>[2x]MNILKHFPSYVGPSKIRTLVIPIGHWTRKEFNNAVQKLSEFNEIHLSDVTPIDSPIFTPQGFPHGKLFFDFLTIDHDDALELFLYDFEPFRKTFVIIGLVNDYSDPLTNLNFMKEKYPTLISPNLVYASSTPTKELEQTIDTMENVFASSPDMQKNIETIMCDIARNFLTALNSYYSSYKHVTLRSPGAIGGNAVLKTTLIRQNSYTSSSSSTPMSAVQSSVSSSSKAGSVTTASKRLSSFEMTTNSLKRSASLKLATTLSTSENRSQQKSLGRQMKILGNFQLLAGRYVDALNSFVDAITTLYKVRDYLWLGSALDGISICFLLLSYLGLSYQIPQIVSLICPVEKLNFESSSTGISPVDSNSKATASTTASSTPRNSISIAAMQSPRNSIMSLSAPALNIDVENINLPLLIKCISDKVLYYYDLSLMHNSEYAPQVVYCEFLLKTLTFMTSCYKSSEFSKDVLDNIVKNQHRALSDIPNSPMFPRFEVYFYSNKLFELQLKEMQVEAQIKIYSTMAEVYRLLGYKRKQLFVLRLLMVALLATPNKIAWHPDYRTLIDTIIELLNINESEAKINVDDPSQSTWLILQKKILQLCIKVSRKINDFEYVAKFSSILITKYTHLLNQSEQDALFKEYIQPSITNESITSYWDPFILREVVINRILDSDPTSNEIPLESDVSSLESLENRQKTQDINPQEVFNPFKRVQPTSFVSNNSTKVPILVFLVGDKAEFTCRVQNPFKFDFTINDIQLDEEISEFCEIDRKAVSYSGPYNVKAESIRSITLPLIIKKPTYKKIYEISCLKISILKLPLQKFDIINDSRRSNPVEEEAEYSKCIYGKLKIKILPEQPQLELLSTSKMTRNSWMMLDGTKTDFHITVRNKSLSCAINHIKIIPMNNIEQMLKPDYWKKMPPDDLYIMEKQLDWLSKSCVRIIKLPTVIKPNETITFDLELDNTAVPFNFTGFDLLIEYGMSATDESCIYLKKLSIPYEVTLRRTIEVPSMDIIPLNELFSSQVENVDWIEYVMSKIRAESNLHSRDFILLLLDFRNSWIDGIKLNVQFEDFTSNEYHVEASHTSRIIVPIKKIDYKKYNFENTPIPRIYPGRQFIQSGLNEEQTIEMRQKFWCREHIISKLKCNWKLTTDQSVTGSVDFNKFIEKFDHKMVYTIYPGRLFYGVQLLLDEPKVKVGEIINLKIITEPTSTCRRKQNSTVNFLDIVIFDSKTSKILPRSNRRILYNGSLTKPISTTKVSEINLEIIPIEKGRYEFSVCISKSNNQDGIIQFDSENVILSVI;>MDKEIYCGSVPVSYFDPFDLFESLRPEFQQILPLDNIHWKAFDGTVRTVNRLPIELIPEGRGEADKSNDEQPFIRFLIVNCISIDQYRAKVRPLVRQWLPNLESVSSSTGEKMIYKPIILLYANSEVVDSNLFKSVSLMEKFGKDFPHVQTLEVRSVYRSPKERQEFWNQFSQKIKASVLSIFQKRLTHLQHSLANLQKGNNFEEQLLTREKLYELYVVFNILEDASLELQKIKKEILRRNMNMPDGKLQVPFESSSKSDESLGSIIIEGTLDKFQLHKYFFIRRLRLLKLEDQTLTAFVGAFQLIKNFIESISIEYRKSVRLLEFKHYFITSMLSYFEFENVSNPLLCEIKAELLMLKRDNWVQGVMATSGYRLMDKNYPNSDVKYKFDLLKETFVDETVFQENFLTLTKEILSLFNKCEGKRQRIVDILSIEIGLLYYQGKKYEEAVSLFLSCYEYYTQTNWNSIGLKILQVFIDSLSHCPKLDVLQIDGESVSASAVLTNAFLNILKLCKDNDSKEIWWKKFMDLQMKNNIHLMYPLDGLFEVTLNSKVHLARANVSAIEVNLKSYGFPEDISTKTMRLSLKNMGGDVIVFGASDFLLKKGENKLILECRDIMYGEFSLLSFEIIVEGITFVKEFPENQDEFIVVPEIYCKESTKVLVKQAHNLNLGEYALELKSVQSDALESLQVEVEVQKNIGNMKNLPVSFSMDEIQARKRYNTPFENVRLEYYLLDQITAFDLIIKTSFTKKNDQGTFGETKKVRIQCYLQLSVSVEDIFKKDIFFFKFLLNSSVREEPVILYSSELSAPDTRNDYNIRGDYIATTPALITFDGNESFINCYEITANNNFDSKDIFNLKVRYNTLKEQLDCFITDAVLIEGDVEWFILFEKWKTFWELEILKKLKYDYDAFKENRIIRLLKTSIDLNKTKSKIRNLCIEKAVLDKILICLNKVSRGIAVCNTDMDEYVRNLVPKQLTVPVQLPGFEQFFHVQFEQMETSHDALHDTIATIGNSLSYTVIVENLSGQWGQDVIDDGGYIFEILSSNEWLIHGQKRCAIKEKRKEFEVHLIPLKKGYLNFPRVEITNINGKSCRVDHSNAFESILIFAA[2x];>[2x]MECFVPLRCDLDGSNIEQLRQSHLSRKFIIFDEQLNLWLWFQGNSQENKRFVLQNMIILINEAQVTRTSTIDDYFTQVENNENLWRLKNDCCSKILFKSNVVMNNGYNNQIKFVFEYKSVDANFNNQDSLQDPQAKYTLDKYSSEEILPSFEPVYSWSSAATKSSKNTNNHLEKNNRATHRVSSKNSEVHEADVSRNPNTFTLKLQYPIFSLLNMRLRNISLKSEHCILSSLDFQTSKASEQLTKKFIYPQEHNSFLKLNFQEISYKLIDGTSQIELDPICPLKVPLTAFSYDSISATFKLVLLPKSTQPHRVKITLAYELELHPNLKLPVRTSWETEVTLKRSMPISSTSSQYSSNNNNTNHSASFNGAANNVNSGGLANLRLGGVSSSRFSLGAASTTSLVNSKLSNVKFKFINSNIKVIKGEKFTMRLQIINSSSSPLDLVVYYNNTINPIPSANNVRNSNGINNCGMNNGTIPNSPLTLENQYQLHNKYRKIAEGIILLSNDYKIPVVPPRETYFADLRFIGIMSGYYGTLSGLKVLDLNTNELIEVGNGASVLIQ;>MSLRPCFVSLIDESDKPILIYVPNEAENEMNDVLKYNVLSNISLDYFESALVEWHSLDSKPLLKSIFQLEGVSVFAMLIKQTGLKIVIGFEQKSLSGADDEFEAINQIFETVRKIYIRVKCNPLLVSGDEKSIIKSLERKFDELFISTEVEL[2x];>[2x]MSSTHSNNVGHPQSSPQGPLTEQQRAQQQYQIFENSLPKVSQSVYQMLLNEMVPLAMGIERQISGDVISSDSNVTSENGNINNMIKRLKIEEHHTVDIIRSHNLIHELYKADEEEKEKVLARLRNIGFQIGLKLSELLIFSNNPNLKFKEMDLLLIMKFICRDVWKQIFGKQIDNLKTNHRGTFYLLDYDYRPIQSFSLEEDAKNEELKMIEPFLEIPVGIIRGVLSSLGYSSEEVICLASFIDRPTDRPKTAFPKGVSFHVQVTMPQ;>MVSTTQSRSLKAMGEEIWKNKTEKINTELFTLTYGSIVAQLCQDYERDFNKVNDHLYSMGYNIGCRLIEDFLARTALPRCENLVKTSEVLSKCAFKIFLNITPNITNWSHNKDTFSLILDENPLADFVELPMDAMKSLWYSNILCGVLKGSLEMVQLDCDVWFVSDILRGDSQTEIKVKLNRILKDEIPIGED[4x];>[2x]MGIYSFWIFDRHCNCIFDREWTLASNSASGTINSKQNEEDAKLLYGMIFSLRSITQKLSKGSVKNDIRSISTGKYRVHTYCTASGLWFVLLSDFKQQSYTQVLQYIYSHIYVKYVSNNLLSPYDFAENENEMRGQGTRKITNRNFISVLESFLAPMVNQ;>[2x]MAIETILVINKSGGLIYQRNFTNDEQKLNSNEYLILASTLHGVFAIASQLTPKALQLTQQTNIENTIPYIPYVGMSSNRSDTRNGGGNNNKHTNNEKLGSFKGDDFFKEPFTNWNKSGLRQLCTDQFTMFIYQTLTGLKFVAISSSVMPQRQPTIATTDKPDRPKSTSNLAIQIADNFLRKVYCLYSDYVMKDPSYSMEMPIRSNLFDEKVKKMVENLQ;>[2x]MSQRIIQPSASDQQFPGKSDGYEYTVGPKQAITSEASTTYIPSRIYSESLLFKRQEASLSAMAFLFQEMISQLHRTCKTAGDFETKLSDYGHNIGIRLLELLNFRASVSPSSLPRASAFLSQNESSSKLSNASNSPGMLANSSTATSASANERLQEKQTESLSNYITKMRRRDLKILDILQFIHGTLWSYLFNHVSDDLVKSSERDNEYMIVDNFPTLTQFIPGENVSCEYFVCGIIKGFLFNAGFPCGVTAHRMPQGGHSQRTVYLIQFDRQVLDREGLRFG;>MPQYFAIIGKKDNPVYEIEFTNAENPQGFPQDLKELNPFILHASLDIVEDLQWQINPTSQLNGNGGNGSNGGGGFLRSRAVNNTDNCYLGKVDHFYGLAITAYISYSGMKFVMIHGNSANSSVVIDDNNMRSFYQEVHELYVKTLMNPFYKITDPIRSPAFDSRVRTLARKHLSK[2x];>[2x]MSNEDYGYDYDYLFKIVLIGDSGVGKSNLLSRFTTDEFNIESKSTIGVEFATRTIEVENKKIKAQIWDTAGQERYRAITSAYYRGAVGALIVYDISKSSSYENCNHWLTELRENADDNVAVGLIGNKSDLAHLRAVPTDEAKNFAMENQMLFTETSALNSDNVDKAFRELIVAIFQMVSKHQVDLSGSGTNNMGSNGAPKGPTISLTPAPKEDKKKKSSNHHHHHHH

There are at least three reported GEFs for Rab11 (3, 11–15); the Rab11 GEF distributed most broadly throughout the eukaryotic kingdom appears to be the multisubunit transport protein particle II (TRAPPII) complex. Yeast TRAPPII comprises 22 subunits encoded by 10 genes, and yeast have two Rab11 paralogs, named Ypt31 and Ypt32. Each of the 11-subunit monomers forms a triangle shape in which the TRAPP core subunits appear to be grasped by tongs composed of the TRAPPII-specific Trs120 and Trs130 subunits. We describe two different conformations of TRAPPII: an open state that allows Rab11 to access the active site chamber and a closed state in which the Trs120 lid encloses the chamber to enable Rab11 activation.

TRAPPII monomers bound to Rab11 adopted only the closed conformation. Viewed from the “side,” each monomer forms a chamber in which Rab11 is sandwiched between the core and Trs120. Superposition of the published structure of inactive, guanosine diphosphate (GDP)–bound Rab11/Ypt32 (37) onto the nucleotide-free activation intermediate indicates that the GTPase “switch I” region has undergone a marked opening concomitant with nucleotide release. As found for Rab1/Ypt1, Rab11/Ypt32 makes contact with the Bet3, Bet5, Trs31, and Trs23 subunits, and we observed density corresponding to the C terminus of one of the Bet3 subunits interacting with the opened nucleotide-binding site. Somewhat unexpectedly, we observed that the HVD of Rab11/Ypt32 binds to the same pocket on the Trs31 core subunit that binds to the HVD of Rab1/Ypt1 in TRAPPIII. The structure of the TRAPPII-Rab11/Ypt32 activation intermediate supports this proposal, as we now observe that Trs120 makes multiple direct contacts with Rab11/Ypt32 on a surface of the GTPase that is distal to its interaction with the core. We identified three different ordered loops of Trs120 that contact Rab11. One of these loops (“loop 1”) interacts with Rab11/Ypt32 by adopting a β strand that binds to the edge of the GTPase β sheet. The other loops (“loop 2” and “loop 3”) make primarily electrostatic interactions with Rab11/Ypt32. In the closed state, nucleotide-free Rab11 is tightly sandwiched in between the TRAPP core and the Trs120 lid, suggesting that conformational change is necessary to enable Rab11 to diffuse into or out of the TRAPPII active site.(4S,5R)-4,5-bis(4-chlorophenyl)-2-methyl-4,5-dihydro-1H-imidazole | C16 H14 Cl2 N2 | 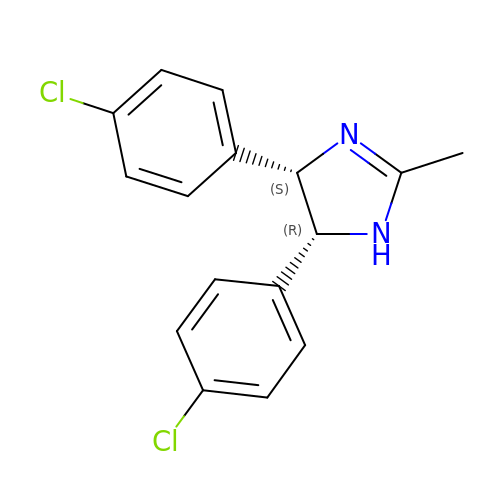VLUCXJXOZXEFPA-IYBDPMFKSA-N> XSMSDVAIVKEGWLHKRGKYIKTWRPRYFLLKNDGTFIGYKERP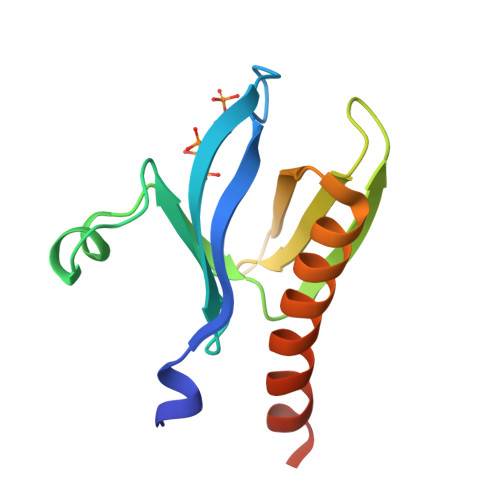QDVDQREAPLNNFSVAQCQLMKTERPRPNTFIIRCLQWTTVIERTFHVETPEEREEWTTAIQTVADGLKKQEEEEMDFRSG>[2x]MIAGSMVALVTPFDAQGRLDWDSLAKLVDFHLQDGTNAIVAVGTTGESATLDVEEHIQVVRRVVDQVKGRIPVIAGTGANSTREAVALTEAAKSGGADACLLVTPYYNKPTQEGMYQHFRHIAEAVAIPQILYNVPGRTSCDMLPE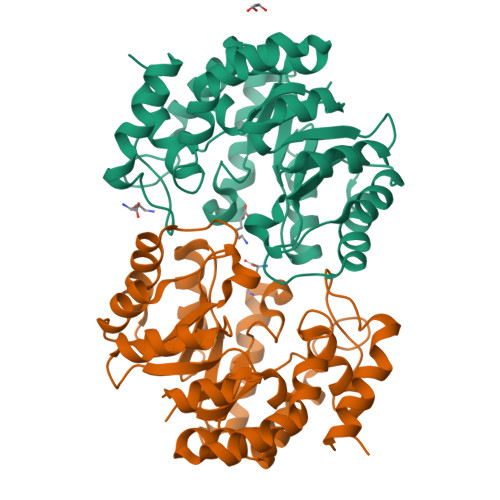TVERLSKVPNIIGIKEATGDLQRAKEVIERVGKDFLVYSGDDATAVELMLLGGKGNISVTANVAPRAMSDLCAAAMRGDAAAARAINDRLMPLHKALFIESNPIPVKWALHEMGLIPEGIRLPLTWLSPHCHDPLRQAMRQTGVLA> MMDLRNTPAKSLDKFIEDYLLPDTCFRMQINHAIDIICGFLKERCFRGSSYPVCVSKVVKGGSSGKGTTLRGRSDADLVVFLSPLTTFQDQLNRRGEFIQEIRRQLEACQRERAFSVKFEVQAPRWGNPRALS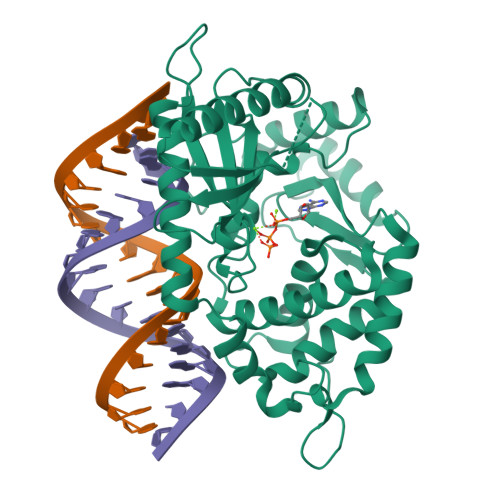FVLSSLQLGEGVEFDVLPAFDALGQLTGGYKPNPQIYVKLIEECTDLQKEGEFSTCFTELQRDFLKQRPTKLKSLIRLVKHWYQNCKKKLGKLPPQYALELLTVYAWERGSMKTHFNTAQGFRTVLELVINYQQLCIYWTKYYDFKNPIIEKYLRRQLTKPRPVILDPADPTGNLGGGDPKGWRQLAQEAEAWLNYPCFKNWDGSPVSSWILLAGP> DEHKAHKAILAYEKGWLAFSLAMLFVFIALIAYTLATHTAGVIPAGKLERVDPTTVRQEGPWADPAQAVVQTGPNQYTVYVLAFAFGYQPNPIEVPQGAE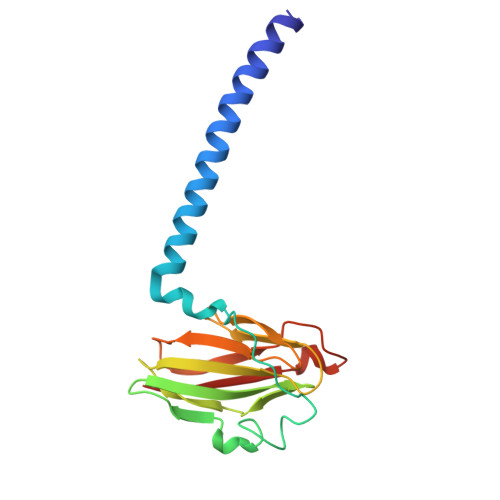IVFKITSPDVIHGFHVEGTNINVEVLPGEVSTVRYTFKRPGEYRIICNQYCGLGHQNMFGTIVVKE>MAEQDLTMIVGTYTSGDSKGLYSFRFNEENGTATALSEAEVENPSYLVPSADGKFIYAVSEFSNEQAAANAFAFNKEEGTFRLLNTQKTGGEDPCYIITNGSNVVTANYSGGSISVFPIDKDGSLLPASEVVKFKGSGADKERQEKPHLHCVRITPDGKYLFADDLGTDQIHKFIVNPNAKADNEDVFLKEGSPASYKVEAGSGPRHLTFAPNGSYAYLINELSGTVIAFEYNDGELKEIQTIAADTVGAKGSGD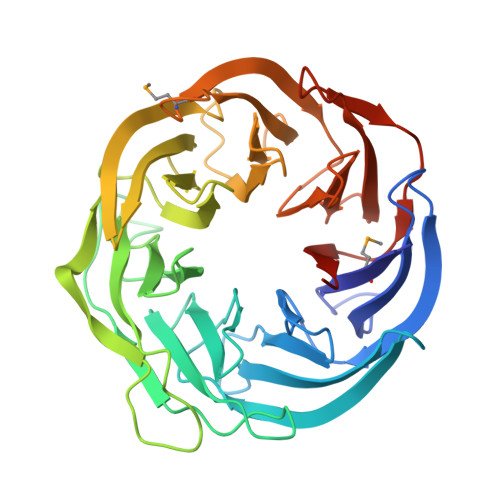IHISPDGKFLYASNRLKADGLAIFSIHPENGMLTKVGYQLTGIHPRNFIITPNGKYLLVACRDSNVIQVYERDTDTGLLTDIRKDIKVDKPVCIKFVPLEHHHHHH[2x]> TVKSLAAAEQWEPSPLTLKQHQQVVVWKKDRTCILCKKEVQGG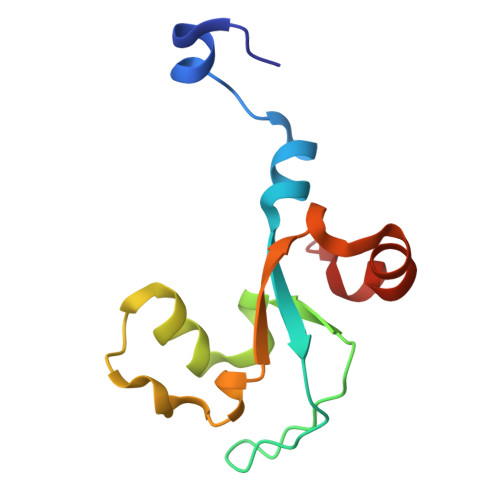NVEKVETACEKAWRFLSGYSRSAHVCPILPQMRILRYGELPLRDRAKFDAKLRRE>[3x]SNAMKILFIGESWHIHMIHSKGFDSFTSSKYEEGADYLLSCLRQGNIDVDYMPAHIVQTRFPQTAEALACYDAIVISDIGSNTFLLQNRTFY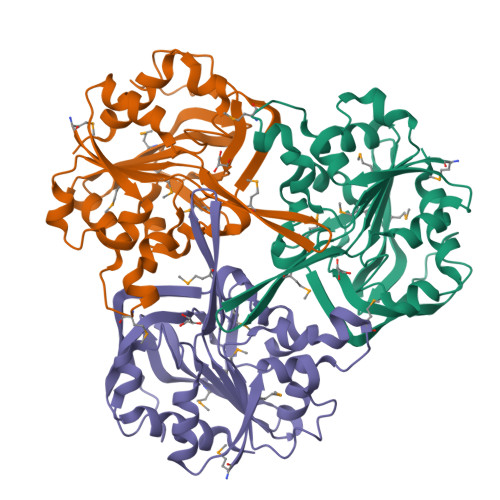NMDIIPDALQLIADYVAEGGGLLMIGGYLSFTGIEAKANYKNTVLAEVLPVDMLDVDDRVELPQGCKAVNTAVEHVITQPFSEWPPLLGYNKLIAKENSQVLAEINGDPLLVMGTYHKGKVCCFASDCSPHWGSPQFLQWEHYATFWCNVLHTIKK> MTKSELIERLATQQSHIPAKTVEDAVKEMLEHMASTLAQGERIEIRGFGSFSLHYRAPRTGRNPKTGDKVELEGKYVP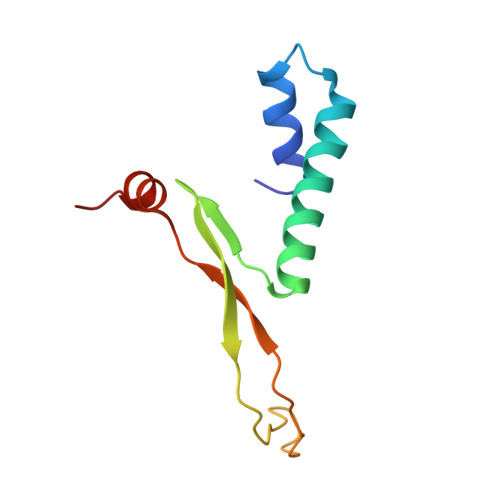HFKPGKELRDRANIYG>SEQNTPLGGCILADTPITFNENKPVTKVKVRNTGDRPIQVGSHFHFFEVNRALEFDRAAAYGKRLNISSTTAIRFEPGDETEVPLIPFGGKQTLYGFNNLVDGWTGEGVVPNSERPDKLEAIRRAAERGFKS[12x];>PQISRQEYAGLFGPTTGDKIRLGDTNLFIEIEKDLRGYGEESVYGGGKSLRDGMGANNHLTRDNGVLDLVITNVTIVDARLGVIKADVGIRDGKIAGIGKSGNPGVMDGVTPGLVVGVSTDAISGEHLILTAAGIDTHIHLISPQQAYHALSNGVATFFGGGIGPTDGTNGTTVTPGPWNIRQMLRSVEGLPVNVGILGKGNSYGRGPLLEQAIAGVVGYKVHEDWGATANALRHSLRMADEMDIQVSVHTDSLNECGYVEDTIDAFEGRTIHTFHTEGAGGGHAPDIIRVASQPNVLPSSTNPTLPYGVNSQAELFDMIMVCHNLNPNVPADVSFAESRVRPETIAAENVLHDMGVISMFSSDSQAMGRVGENWLRVMQTANAMKASRGKLPEDAPGNDNFRVLRYVAKITINPAIAQGVSHVIGSVEVGKMADLVLWDPRFFGAKPKMVIKGGMINWAAMGDPNASLPTPQPVFYRPMFGAMGKTMQDTCVTFVSQAALDDGVKEK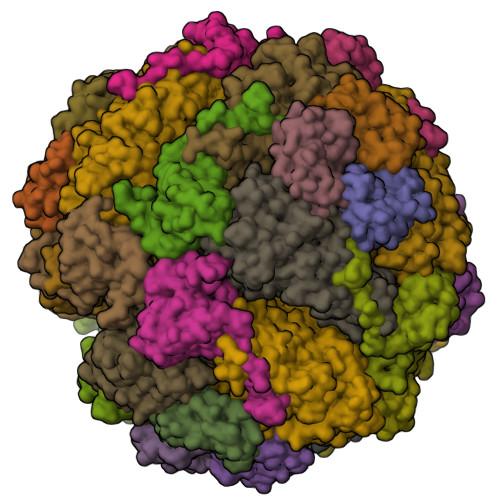AGLDRQVIAVKNCRTISKHDLVRNDQTPNIEVDPETFAVKVDGVHATCEPIDTAAMNQRYFFG[12x];>[12x]MQLTPREVEKLMIYTLSDVAFKRKARGLKLNYPEAVSIITVTAMEGARDGKSVEDVMKEASKVLTKDDVMDGVADLIPNVQVEAIFTDGSRLVTVHDPIK> MAHHHHHHMNNADAQLATCYGPVSQAFVDRAAKIRLLILDVDGVLSDGLIYMGNHGEELKAFNVRDGYGIRCALTSGIEVAIITGRKAKLVEDRCQTLGITHLYQGQSDKLLAFRDLTDKLHVRPEEVAYIGDDLIDWPVMAEVGLSVAVADAHPLLLPRANYVTRINGGR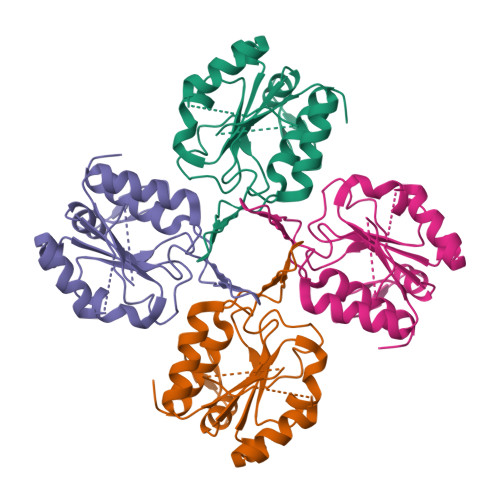GAVREVCDLLLLAQGKLDEAKGQSI>MASGMIVTDAGADQPIVFVNRAFSTITGYAPNEVLGRNARFLQGPQTDAATVARLREAIAAARPIQERILNYRKDGQPFWNQLSISPVRDETGNVVAFVGVETD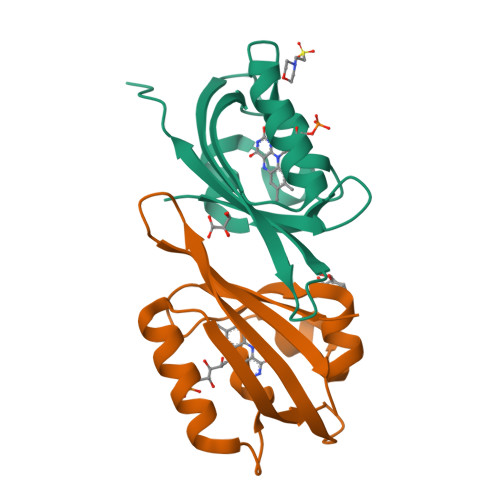VTAHHHHHH[2x]> QTQDPLYGYFAAVAGQDGQIDADELQRCLTQSGIAGGYKPFNLETCRLMVSMLDRDMSGTMGFNEFKELWAVLNGWRQHFISFDTDRSGTVDPQELQKALTTMGFRLSPQAVNSIAKRYSTNGKITFDDYIACCVKLRALTDSFRRRDTAQQGVVNFPYDDFIQCVMSV

Sorcin (Soluble resistance-related calcium binding protein) is a calcium binding oncoprotein expressed at high levels in several human tumours, such as leukaemia, gastric, breast and ovarian cancers. Each monomer of Sorcin homodimer is formed by two domains, i.e. a flexible, glycine-rich N-terminal domain and a C-terminal calcium-binding domain (SCBD), endowed with five EF-hands3031. The SCBD can be divided in two regions: EF1–3 (residues 33–134), which binds calcium with high affinity, and EF4–5 (residues 135–198), which mediates dimerization. Upon calcium binding Sorcin undergoes a large conformational change that allows it to bind and regulate a series of target proteins in a calcium-dependent fashion.

To investigate the structural basis of Sorcin activation and of selective calcium-dependent signal transduction, we here solved the structure of the apo Sorcin (apoSor) and, for the first time, the structure of Sorcin in the calcium-bound form (CaSor). Briefly, the monomer is formed by two domains: a Gly-rich N-terminal domain (residues 1–32), partially visible in both apo and calcium-bound structures (residues 30–32 and 26–32, respectively), and a calcium binding domain (SCBD), containing eight α-helices (A-H) organised in five calcium binding motifs (EF1-EF5). Indeed, the rmsd values measured by superimposing CaSor to the apoSor clearly indicate that upon calcium binding Sorcin undergoes a large conformational change, mainly involving EF1, EF2 and EF3. The comparison between apoSor and the calcium-bound Sorcin structures sheds light on the mechanism of cation-mediated structural changes of Sorcin, which is fundamental for the comprehension of its function. The residues with a difference in SASA (Solvent Accessible Surface Areas) higher than 30% between the apo and the calcium bound form of Sorcin are Tyr67, Ser80, Met81, Met86, Ile110, Arg116, Gly118, Ser143 and Ser197. Tyr67 is placed on the loop between helices B and C, and in apoSor it is hydrogen bonded to Asp113 of the EF3 loop and is partially covered by it. Upon calcium binding this interaction is broken since Asp113 participates in ion coordination; the rearrangement of the EF3 loop causes also the exposure of Arg116. The superimposition between the CaSor and apoSor shed light on the mechanism of Sorcin activation induced by the calcium binding to EF3: the binding of the cation promotes the movement of three calcium ligands (Asp113, Asp115 and Ser117) towards the E-helix where Glu124, the bidentate ligand, is located and consequently, a large movement of the D helix with respect to the E helix (about 15°). This movement is transmitted to the EF1-EF2 subdomain via the Tyr 67 placed in a strategic position, in the middle of the loop connecting EF1 to EF2, and anchoring the EF1-EF2 subdomain to the EF3 loop.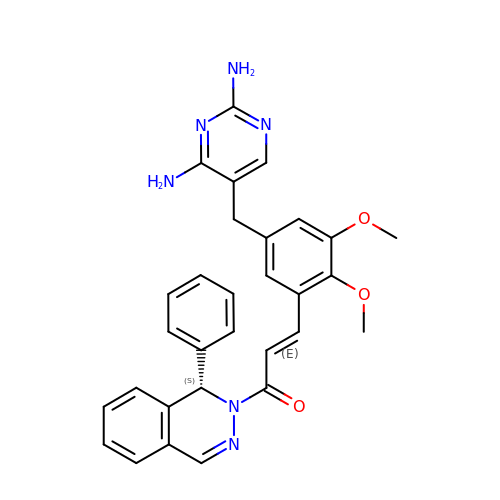(2E)-3-{5-[(2,4-diaminopyrimidin-5-yl)methyl]-2,3-dimethoxyphenyl}-1-[(1S)-1-phenylphthalazin-2(1H)-yl]prop-2-en-1-one | C30 H28 N6 O3 | NFQBNKYRVDDBSW-QSRYBZNWSA-N> GSHMASMTGGQQMGRGSMGNLMISFLKKDTQSITLEELAKIIKKCKHVVALTGSGTSAESNIPSFRGSSNSIWSKYDPRIYGTIWGFWKYPEKIWEVIRDISSDYEIEINNGHVAL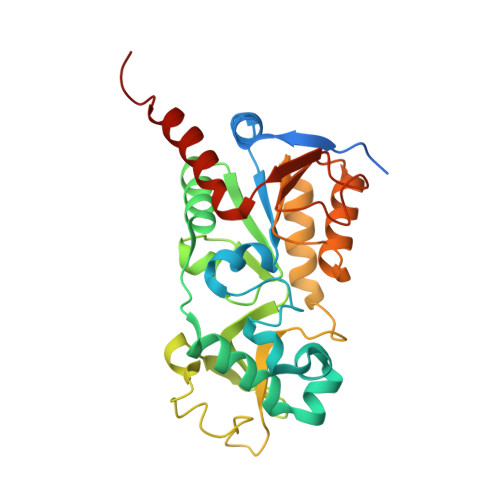STLESLGYLKSVVTQNVDGLHEASGNTKVISLHGNVFEAVCCTCNKIVKLNKIMLQKTSHFMHQLPPECPCGGIFKPNIILFGEVVSSDLLKEAEEEIAKCDLLLVIGTSSTVSTATNLCHFACKKKKKIVEINISKTYITNKMSDYHVCAKFSELTKVANILKGSSEKNKKIM> MSKLEAILSQEVEAEIQALLQEAE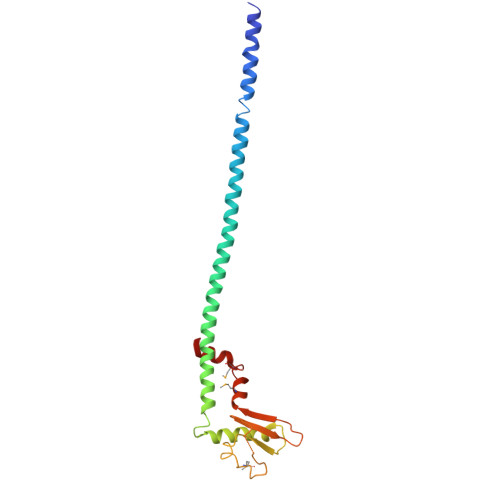AKAEAVKREAEEKAKALLQARERALEAQYRAALRRAESAGELLVATARTQARGEVLEEVRRRVREALEALPQKPEWPEVVRKLALEALEALPGAKALVANPEDLPHLEAMARERGVELQAEPALRLGVRAVGAEGKTQVENSLLARMDRAWDAMSSKVAQALWG> MANELTWHDVLAEEKQQPYFLNTLQTVASERQSGVTIYPPQKDVFNAFRFTELGDVKVVILGQDPYHGPGQAHGLAFSVRPGIAIPPSLLNMYKELENTIPGFTRPNHGYLESWARQGVLLLNTVLTVRAGQAHSHASLGWETFTDKVISLINQHREGVVFLLWGSHAQKKGAIIDKQRHHVLKAPQPSPLSAHRGFFGCNHFVLANQWLEQHG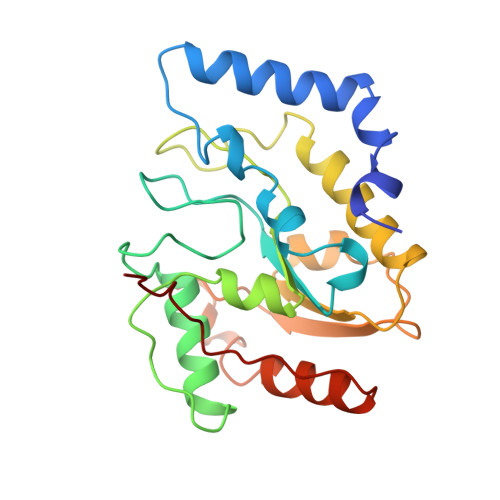ETPIDWMPVLPAESE>[2x]MGHHHHHHHHHHSSGHIDDDDKHMHNDKDLSTWQTFRRLWPTIAPFKAGLIVAGVALILNAASDTFMLSLLKPLLDDGFGKTDRSVLVWMPLVVIGLMILRGITSYVSSYCISWVSGKVVMTMRRRLFGHMMGMPVSFFDKQSTGTLLSRITYDSEQVASSSS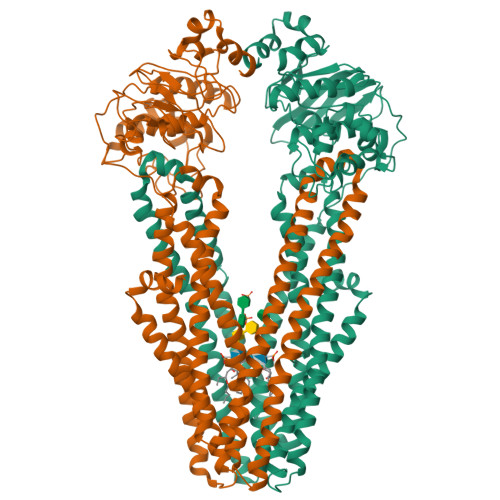GALITVVREGASIIGLFIMMFYYSWQLSIILIVLAPIVSIAIRVVSKRFRNISKNMQNTMGQVTTSAEQMLKGHKEVLIFGGQEVETKRFDKVSNRMRLQGMKMVSASSISDPIIQLIASLALAFVLYAASFPSVMDSLTAGTITVVFSSMIALMRPLKSLTNVNAQFQRGMAACQTLFTILDSEQEKDEGKRVIERATGDVEFRNVTFTYPGRDVPALRNINLKIPAGKTVALVGRSGSGKSTIASLITRFYDIDEGEILMDGHDLREYTLASLRNQVALVSQNVHLFNDTVANNIAYARTEQYSREQIEEAARMAYAMDFINKMDNGLDTVIGENGVLLSGGQRQRIAIARALLRDSPILILDEATSALDTESERAIQAALDELQKNRTSLVIAHRLSTIEKADEIVVVEDGVIVERGTHNDLLEHRGVYAQLHKMQFGQ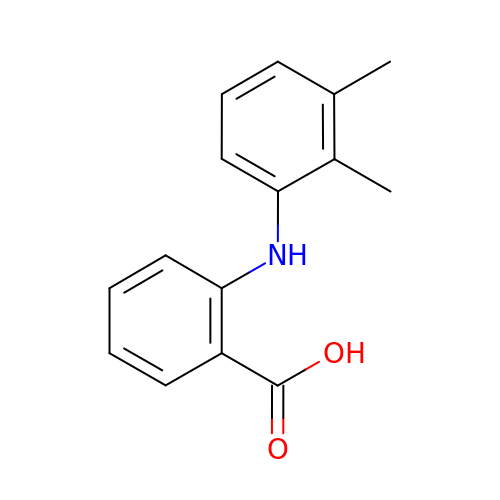2-[(2,3-DIMETHYLPHENYL)AMINO]BENZOIC ACID | C15 H15 N O2 | HYYBABOKPJLUIN-UHFFFAOYSA-N> PISPIETVPVKLKPGMDGPKVKQWPLTEEKIKALVEICTEMEKEGKISKIGPENPYNTPVFAIKKKDSTKWRKLVDFRELNKRTQDFWEVQLGIPHPAGLKKKKSVTVLDVGDAYFSVPLDEDFRKYTAFTIPSINNETPGIRYQYNVLPQGWKGSPAIFQSSMTKILEPFKKQNPDIVIYQYMDDLYVGSDLEIGQHRTKIEELRQHLLRWGLTTPDKKHQKEPPFLWMGYELHPDKWTVQPIVLPEKDSWTVNDIQKLVGKLNWASQIYPGIKVRQLCKLLRGTKALTEVIPLTEEAELELAENREILKEPVHGVYYDPSKDLIAEIQKQGQGQWTYQIYQEPFKNLKTGKYARMRGAHTNDVKQLTEAVQKITTESIVIWGKTPKFKLPIQKETWETWWTEYWQATWIPEWEFVNTPPLVKLWYQLEKEPIVGAETFYVDGAANRETKLGKAGYVTNKGRQKVVPLTNTTNQKTQLQAIYLALQ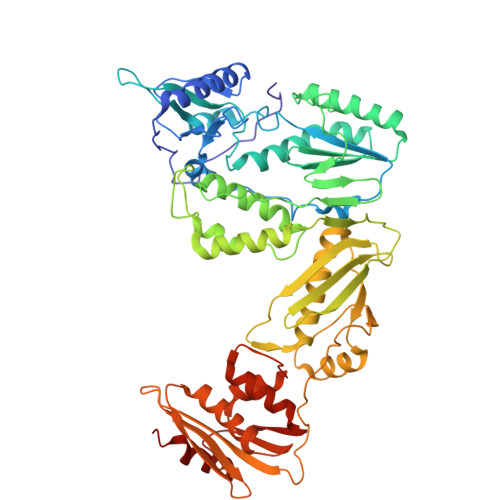DSGLEVNIVTDSQYALGIIQAQPDKSESELVNQIIEQLIKKEKVYLAWVPAHKGIGGNEQVDKLVSAGIRKIL>MRTRSTISTPNGITWYYEQEGTGPDVVLVPDGLGECQMFDSSVSQIAAQGFRVTTFDMPGMSRSAKAPPETYTEVTAQKLASYVISVLDALDIKHATVWGCASGASTVVALLLGYPDRIRNAMCHELPTKLLDHLSNTAVLEDEEISKILANHMLNDVSGGSEAWQAMGDEVHARLHKNYPVWARGYPRTIPPSAPVKDLEALRGKPLDWTVGAATPTESFFDNIVTATK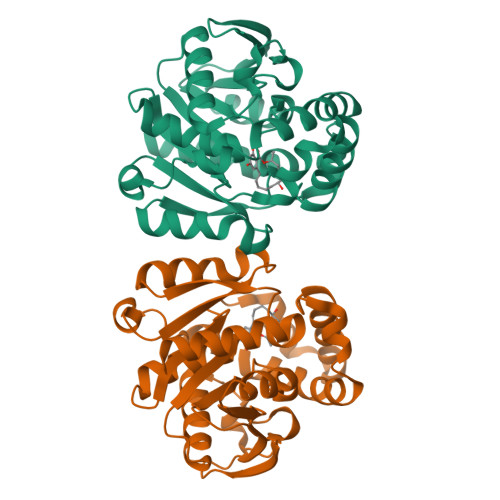AGVNIGLLPGMHFPYVSHPDVFAKYVVETTQKHL[3x]> GAMAGSIRSKLSAIDVRQLGTVDYRTAWQLQRELADARVAGGADTLLLLEHPAVYTAGRRTETHERPIDGTPVVDTDRGGKITWH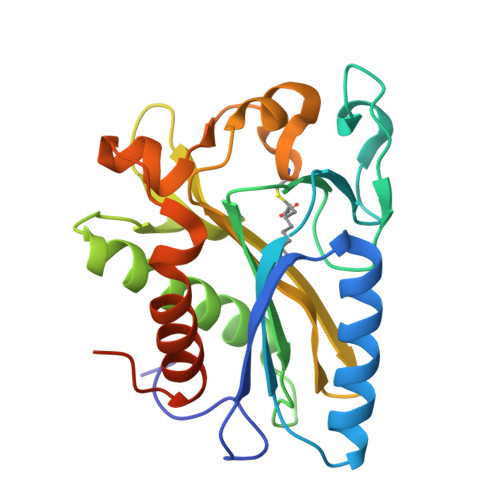GPGQLVGYPIIGLAEPLDVVNYVRRLEESLIQVCADLGLHAGRVDGRSGVWLPGRPARKVAAIGVRVSRATTLHGFALNCDCDLAAFTAIVPCGISDAAVTSLSAELGRTVTVDEVRATVAAAVCAALDGVLPVGDRVPSHAVPSPL> MQRSPLEKASVVSKLFFSWTRPILRKGYRQRLELSDIYQIPSVDSADNLSEKLEREWDRELASKKNPKLINALRRCFFWRFMFYGIFLYLGEVTKAVQPLLLGRIIASYDPDNKEERSIAIYLGIGLCLLFIVRTLLLHPAIFGLHHIGMQMRIAMFSLIYKKTLKLSSRVLDKISIGQLVSLLSNNLNKFDEGLALAHFVWIAPLQVALLMGLIWELLQASAFCGLGFLIVLALFQAGLGRMMMKYRDQRAGKISERLVITSEMIENIQSVKAYCWEEAMEKMIENLRQTELKLTRKAAYVRYFNSSAFFFSGFFVVFLSVLPYALIKGIILRKIFTTISFCIVLRMAVTRQFPWAVQTWYDSLGAINKIQDFLQKQEYKTLEYNLTTTEVVMENVTAFWEEGFGELFEKAKQNNNNRKTSNGDDSLFFSNFSLLGTPVLKDINFKIERGQLLAVAGSTGAGKTSLLMVIMGELEPSEGKIKHSGRISFCSQFSWIMPGTIKENIIFGVSYDEYRYRSVIKACQLEEDISKFAEKDNIVLGEGGITLSGGQRARISLARAVYKDADLYLLDSPFGYLDVLTEKEIFESCVCKLMANKTRILVTSKMEHLKKADKILILHEGSSYFYGTFSELQNLQPDFSSKLMGCDSFDQFSAERRNSILTETLHRFSLEGDAPVSWTETKKQSFKQTGEFGEKRKNSILNPINSIRKFSIVQKTPLQMNGIEEDSDEPLERRLSLVPDSEQGEAILPRISVISTGPTLQARRRQSVLNLMTHSVNQGQNIHRKTTASTRKVSLAPQANLTELDIYSRRLSQETGLEISEEINEEDLKECFF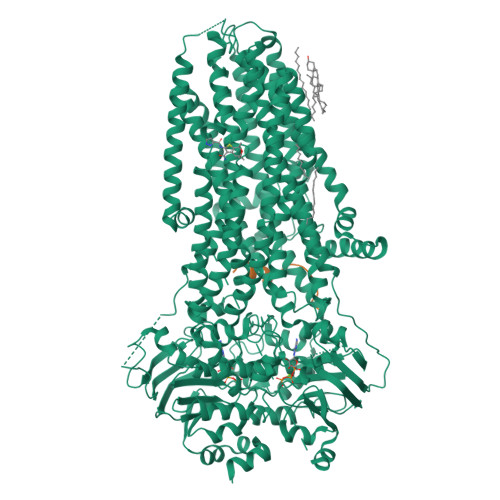DDMESIPAVTTWNTYLRYITVHKSLIFVLIWCLVIFLAEVAASLVVLWLLGNTPLQDKGNSTHSRNNSYAVIITSTSSYYVFYIYVGVADTLLAMGFFRGLPLVHTLITVSKILHHKMLHSVLQAPMSTLNTLKAGGILNRFSKDIAILDDLLPLTIFDFIQLLLIVIGAIAVVAVLQPYIFVATVPVIVAFIMLRAYFLQTSQQLKQLESEGRSPIFTHLVTSLKGLWTLRAFGRQPYFETLFHKALNLHTANWFLYLSTLRWFQMRIEMIFVIFFIAVTFISILTTGEGEGRVGIILTLAMNIMSTLQWAVNSSIDVDSLMRSVSRVFKFIDMPTEGKPTKSTKPYKNGQLSKVMIIENSHVKKDDIWPSGGQMTVKDLTAKYTEGGNAILENISFSISPGQRVGLLGRTGSGKSTLLSAFLRLLNTEGEIQIDGVSWDSITLQQWRKAFGVIPQKVFIFSGTFRKNLDPYEQWSDQEIWKVADEVGLRSVIEQFPGKLDFVLVDGGCVLSHGHKQLMCLARSVLSKAKILLLDQPSAHLDPVTYQIIRRTLKQAFADCTVILCEHRIEAMLECQQFLVIEENKVRQYDSIQKLLNERSLFRQAISPSDRVKLFPHRNSSKCKSKPQIAALKEETEEEVQDTRLSNSLEVLFQ>CGRFAQSQTREDYLALLAEDIERDIPYDPEPIGRYNVAPGTKVLLLSERDEHLHLDPVFWGYAPGWWDKPPLINARVETAATSRMFKPLWQHGRAICFADGWF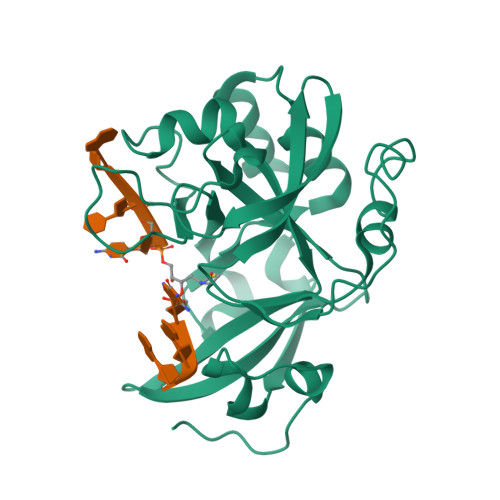EWKKEGDKKQPFFIYRADGQPIFMAAIGSTPFERGDEAEGFLIVTAAADQGLVDIHDRRPLVLSPEAAREWMRQEISGKEASEIAASGCVPANQFSWHPVSRAVGNVKNQGAELIQPVLEVLFQ[2x]>[2x]MKVQYSFEREFEELMSDLLSKYGYEMFQMDGLGDQLDVVKFTEDFVRRGIIEST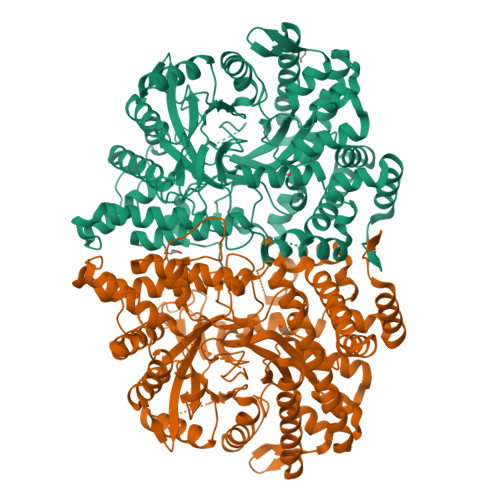IDANANVRVTNISTYFIEISKPHTYLYSLYRIWQKMKEMFGKGVADEFVEAQINGAVYLHDRHHAALMPYCFAYTLKPIVEKGLPFIKTIKSEPAKHLSTFIQHVIQFVMFASNQSSGAVGLPDFFVWMWYFVKKDLKEGIIPRDKLDWYIEQHFQILTYSLNQPIRTTQSPYTNFTYLDRNYIKAIFEGERYPDGSLITDHVEDIIALQKHYWEWVSRERERQMFTFPVLTASLLYKDGKFLDEDSARFINKINMKWQDTNWYISDSIDAVASCCRLTSSTQTLKKFSLSSEEEEKLKGRMNSIGGSDLNIGSFKVITVNLPRIALESGGDREKYLQILRHRVQLIKKALAAVREIIKERISEGLLPLYENGLMLLNRQYGTIGVTGVWESASIMGLTTEDIDGLKYTEEGEVFVDNVLDTIREEAEKGYHEYGFTFNIEQVPAEKAAVTLAQKDRFLFGEKQPFEIYSNQWVPLMANTDVLNRIRYSGKWDKKVSGGAILHINLGESFKTEEESFNMVKMIADMGVMYFAFNTKISVCEDGHAFYGERCPVCGKAKVDEYMRIVGYLVPVSAFNKERREIEYPRRQFYDSLTIRR URIDINE-DIPHOSPHATE-1-DEOXY-1-THIO-N-ACETYLGLUCOSAMINE | C17 H27 N3 O16 P2 S | 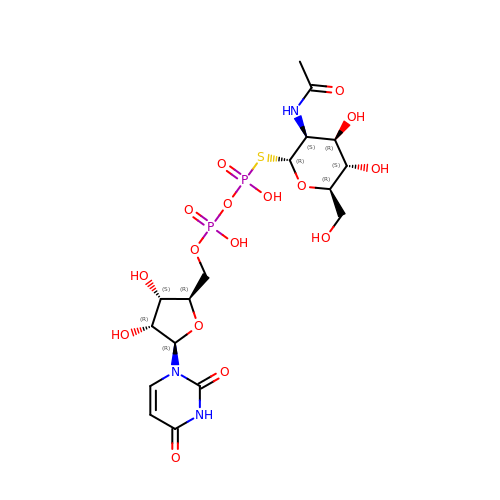NBABRWVWQSKDQY-ZYQOOJPVSA-N> PVAKVEPIKIMLKPGKDGPKLRQWPLTKEKIEALKEICEKMEKEGQLEEAPPTNPYNTPTFAIKKKDKNKWRMLIDFRELNKVTQDFTEIQLGIPHPAGLAKKRRITVLDVGDAYFSIPLHEDFRPYTAFTLPSVNNAEPGKRYIYKVLPQGWKGSPAIFQHTMRQVLEPFRKANKDVIIIQYMDDILIASDRTDLEHDRVVLQLKELLNGLGFSTPDEKFQKDPPYHWMGYELWPTKWKLQKIQLPQKEIWTVNDIQKLVGVLNWAAQLYPGIKTKHLCRLISGKMTLTEEVQWTELAEAELEENRIILSQEQEGHYYQEEKELEATVQKDQDNQWTYKIHQEEKILKVGKYAKVKNTHTNGIRLLAQVVQKIGKEALVIWGRIPKFHLPVEREIWEQWWDNYWQVTWIPDWDFVSTPPLVRLAFNLVGDPIPGAETFYTDGSCNRQSKEGKAGYVTDRGKDKVKKLEQTTNQ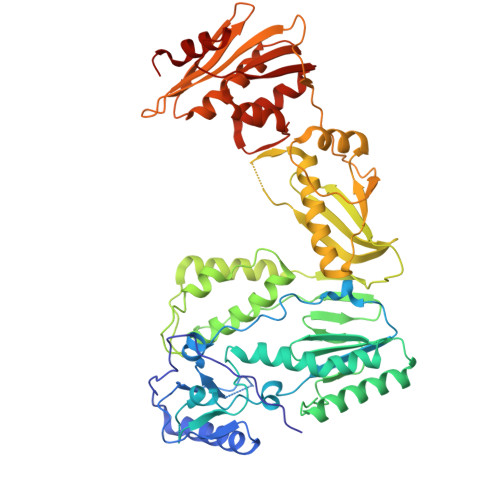QAELEAFAMALTDSGPKVNIIVDSQYVMGIVASQPTESESKIVNQIIEEMIKKEAIYVAWVPAHKGIGGNQEVDHLVSQGI(2S)-4-[2-amino-6-(3-amino-2H-indazol-6-yl)pyrimidin-4-yl]-N-phenylmorpholine-2-carboxamide | C22 H22 N8 O2 | 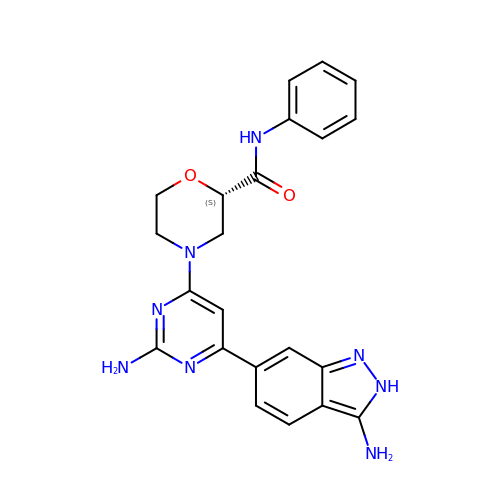NCSQDKMOKNQGSG-SFHVURJKSA-N>GPSQDASDGLQRLHMLQISYFRDPYHVWYQGNASLGGHLTHVLEGPDTNTTIIQLQPLQEPESWARTQSGLQSYLLQFHGLVRLVHQERTLAFPLTIRCFLGCELPPEGSRAHVFFEVAVNGSSFVSFRPERALWQ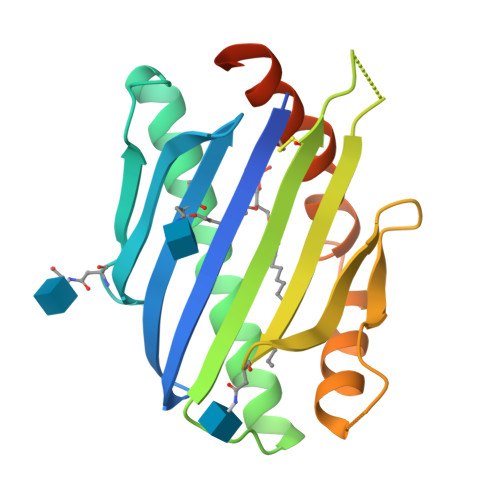ADTQVTSGVVTFTLQQLNAYNRTRYELREFLEDTCVQYVQKHISAENTKGSQTSRSYTS[2x]PaGT3, a uridine diphosphate glycosyltransferase (UGT) from Phytolacca americana, is known for its ability to glycosylate capsaicinoids and other phenolic compounds. PaGT3 adopts a GT-B-fold structure that is highly conserved among UGTs. However, the acceptor-binding pocket in PaGT3 is hydrophobic and large, and is surrounded by longer loops. The larger acceptor-binding pocket in PaGT3 allows the enzyme to bind a range of compounds, while the flexibility of the longer loops possibly plays a role in accommodating the acceptors in the binding pocket according to their shape and size.

We also determined the crystal structure of PaGT3 with UDP-2FGlc and kaempferol at 1.85 Å resolution to understand the poor regioselectivity in the glycosylation of acceptors with multiple possible glycosylation sites. Compared with the apo-PaGT3 structure, the loop Gly78–Gly91 shifts towards the acceptor-binding pocket in the kaempferol-bound structure. The crystal structure of PaGT3 with UDP-2FGlc and kaempferol is similar to the capsaicin-complexed structure, with an r.m.s.d. of 0.34 Å for 855 Cα atoms. The electron density of kaempferol in both molecules of the enzyme clearly indicates that ring A faces towards the inner side of the acceptor-binding pocket. Superposition of the kaempferol molecules in molecules A and B of the enzyme shows that the binding positions of the two kaempferol molecules are different. Interestingly, the 3-OH groups on kaempferol are at distances of 2.6 and 2.9 Å from the catalytic His20 in molecules A and B of PaGT3, respectively. However, the distances between 3-OH of kaempferol and the C1 atom in the 2FGlc moieties of UDP-2FGlc in molecules A and B of PaGT3 are 5.5 and 3.8 Å, respectively. As PaGT3 glycosylates kaempferol to form kaempferol 3-O-glucoside as the major product, the binding orientation of kaempferol in molecule B is likely to be a close representation of the Michaelis complex that forms the major product. The binding of kaempferol in PaGT3 protomers in the asymmetric unit is an indication that sugar-acceptor molecules can bind in different orientations in the acceptor-binding pocket. On the other hand, the binding of kaempferol is assisted by a network of hydrogen bonds provided by water molecules, which could be due to the smaller size of kaempferol compared with the size of the acceptor-binding pocket. The crystal structure of PaGT3 with kaempferol and UDP-2FGlc shows that smaller molecules can bind in different positions/conformations due to the large acceptor-binding pocket of the enzyme.

>[2x]MNHKVHHHHHHLQENLYFQGMGAEPQQLHVVFFPIMAHGHMIPTLDIARLFAARNVRATIITTPLNAHTFTKAIEMGKKNGSPTIHLELFKFPAQDVGLPEGCENLEQALGSSLIEKFFKGVGLLREQLEAYLEKTRPNCLVADMFFPWATDSAAKFNIPRLVFHGTSFFSLCALEVVRLYEPHKNVSSDEELFSLPLFPHDIKMMRLQLPEDVWKHEKAEGKTRLKLIKESELKSYGVIVNSFYELEPNYAEFFRKELGRRAWNIGPVSLCNRSTEDKAQRGKQTSIDEHECLKWLNSKKKNSVIYICFGSTAHQIAPQLYEIAMALEASGQEFIWVVRNNNNNDDDDDDSWLPRGFEQRVEGKGLIIRGWAPQVLILEHEAIGAFVTHCGWNSTLEGITAGVPMVTWPIFAEQFYNEKLVNQILKIGVPVGANKWSRETSIEDVIKKDAIEKALREIMVGDEAEERRSRAKKLKEMAWKAVEEGGSSYSDLSALIEELRGYHA>MHRTSNGSHATGGNLPDVASHYPVAYEQTLDGTVGFVIDEMTPERATASVEVTDTLRQRWGLVAGGAYCA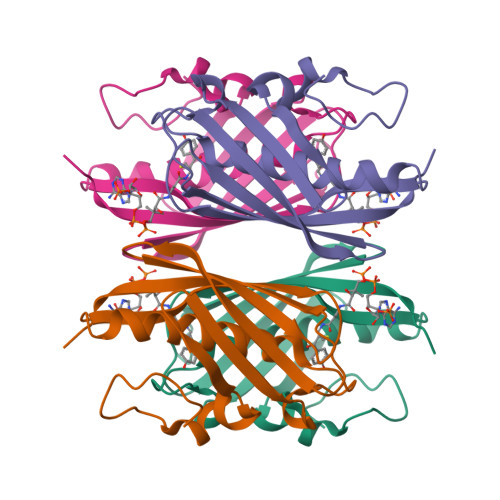LAEMLATEATVAVVHEKGMMAVGQSNHTSFFRPVKEGHVRAEAVRIHAGSTTWFWDVSLRDDAGRLCAVSSMSIAVRPRRD[2x]> EYRNWSKPQCDITGFAPFSKDNSIRLSAGGDIWVTREPYVSCDPDKCYQFALGQGTTLNNVHSNNTVRDRTPYRTLLMNELGVPFHLGTKQVCIAWSSSSCHDGKAWLHVCITGDDKNATASFIYNGRLVDSVVSWSKEILRTQESECVCINGTCTVVMTDGSASGKADTKILFIEEGKIVHTSTLSGSAQHVEECSCYPRYPGVRCVCRDNWKGSNRPIVDINIKDHSIVSSYVCSGLVGDTPRKNDSSSSSHCLDPNNEEGGHGVKGWAFDDGNDVWMGRTISEKSRLGYETFKVIEGWSNPKSKLQ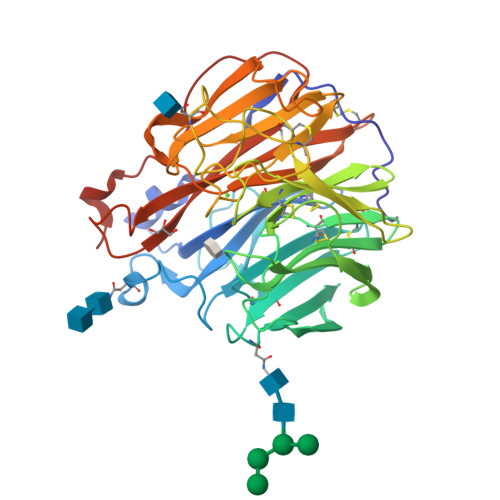INRQVIVDRGNRSGYSGIFSVEGKSCINRCFYVELIRGRKEETEVLWTSNSIVVFCGTSGTYGTGSWPDGADINLMPI>[6x]KLPTNLAYERSIDPSDVCFFVVWPDDRKTPLTYNSRTLLGQMEAKSLAYDVSGQPIKSATAEALAQGNPHQVDFCHVPYGASHIECSFSVSFSSELRQPYKCNSSKVKQTLVQLVELYETKIGWTELATRYLMNICNGKWLWKNTRKAYCWNIVLTPWPWNGEKVGFEDIRTNYTSRQDFKNNKNWSAIVEMIKTAFSSTDGLAIFEVRATLHLPTNAMVRPSQVFTEKETQNSRVFQSTTIDGERSPILGAFKTGAAIATIDDWYPEATEPLRVGRFGVHREDVTCYRHPSTGKDFFSILQQAEHYIEVLSANKTPAQETINDMHFLMANLIKGGMFQHKGD;> LKEIIASNPDDLTTELKRAFRPLTPHIAIDGNEIDALTILVNLTDKAKCKQKLRDEKWWASCINCVNYRQSHNPKFPDIRSEGVIRTQALGELPSFLLSSSKIPPYHWSYSHDSKYVNKSAFLTNEFCWDGEISCLGELLKDADHPLWNTLKKLGCSQKTCKAMAKQLADITLTTINVTLAPNYLTQISLPDSDTSYISLSPVASLSMQSHFHQRLQDENRHSAITRFSRTTNMGVTAMTCGGAFRMLKSGAKFSSPPHHRLNNGSFLVLPNIRVCGATALSSPVTVGIPSLTAFFGFVHAFERNINRTTSSFRVESFAICVHQLHVEKRGLTAEFVEKGDGTISAPATRDDWQCDVVF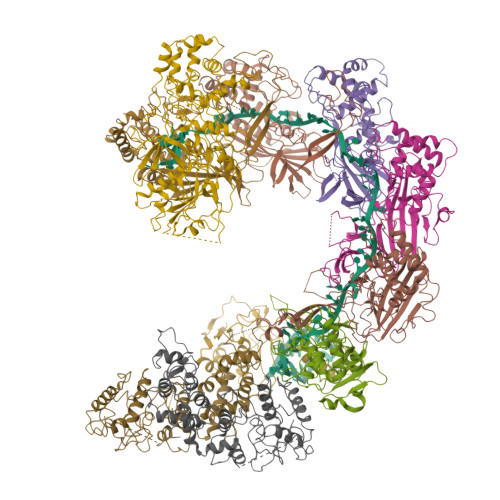SLILNTNFAQHIDQDTLVTSLPKRLARGSAKIAIDDFKHINSFSTLETAIESLPIEAGRWLSLYAQSNNNLSDLLAAMTEDHQLMASCVGYHLLEEPKDKPNSLRGYKHAIAECIIGLINSITFSSETDPNTIFWSLKNYQNYLVVQPRSIN;> KWYYKTITFLPELCNNESLAAKCLRVLHGFNYQYETRNIGVSFPLWCDATVGKKISFVSKNKIELDLLLKQHYFVQMEQLQYFHISNTVLVPEDCTYVSFRRCQSIDKLTAAGLARKIRRLEKRALSRGEAFDPSSFAQKEHTAIAHYHSLGESSKQTNRNFRLNIRMLSEQPREGNSIFSSYGLANSENSFQPVPLI;> AMFLQRPKPYSDESLESFFIRVANKNGYGDVHRFLEATKRFLQDIDHNGYQTFPTDITRINPYSAKNSSSARTASFLKLAQLTFNEPPELLGLAINRTNMKYSPSTSAVVRGAEVFPRSLLRTHSIPCCPLCLRENGYASYLWHFQGYEYCHSHNVPLITTCSGHEAACTVSNWLAGHESKPLPNLPKSYRWGLVHWWMGIKDSDHFSFVQFFSNWPRSFHSIIEDEVEFNLEHAVVSTSELRLKDLLGRLFFGSIRLPERNLQHNIILGELLCYLENRLWQDKGLIANLKMNALEATVMLNCSLDQIASMVEQRILKPNRKSKDVTDYLFHFGDIFCLWLAEFQSDEFNRSFYVSRW;> AMFLQRPKPYSDESLESFFIRVANKNGYGDVHRFLEATKRFLQDIDHNGYQTFPTDITRINPYSAKNSSSARTASFLKLAQLTFNEPPELLGLAINRTNMKYSPSTSAVVRGAEVFPRSLLRTHSIPCCPLCLRENGYASYLWHFQGYEYCHSHNVPLITTCSCGKEFDYRVSEAACTVSNWLAGHESKPLPNLPKSYRWGLVHWWMGIKDDHFSFVQFFSNWPRSFHSIIEDEVEFNLEHAVVSTSELRLKDLLGRLFFGSIRLPERNLQHNIILGELLCYLENRLWQDKGLIANLKMNALEATVMLNCSLDQIASMVEQRILKPNAAAAAAAAADVTDYLFHFGDIFCLWLAAFQSDEFNRSFYVSR> LDFDILTNDGTHRNMKLLIDLKNIFSRQLPKMPKEYIVKLVFDRHHESMVILKNKQKVIGGICFRQYKPQRFAEVAFLAVTANEQVRGYGTRLMNKFKDHMQKQNIEY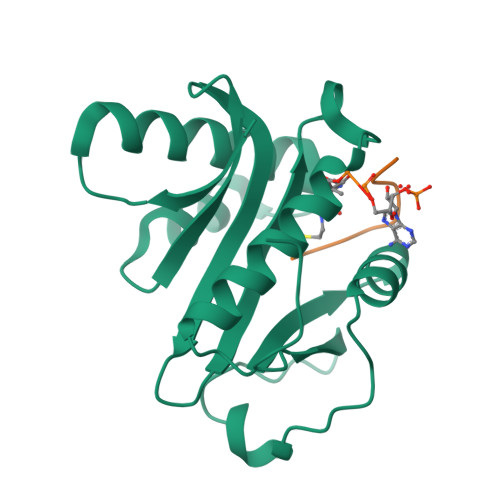LLTYADNFAIGYFKKQGFTKEHRMPQEKWKGYIKDYDGGTLMECYIHPYVDYGR;> SGRGKGGKGLGKGGAKRHR>[2x]MNVTVDQSTLAGATRGIVRGGETLKEHRDRLMAATKATGRYAGLKTLELREREPILYNKLFSRLRAGVVDARETAKKIAASPIVEQEGELCFTLYNAAGDSLLTSTGIIIHVGTMGAAIKYMIENNWEANPGVHDKDIFCNNDSLIGNVHPCDIHTIVPIFWEGELIGWVGGVTHVIDTGAVGPGSMATGQVQRFGDGYSITCRKVGANDTLFRDWLHESQRMVRTTRYWMLDERTRIAGCHMIRKLVEEVVAEEGIEAYWKFAYEAVEHGRLGLQARIKAMTIPGTYRQVGFVDVPYAHEDVRVPSDFAKLDTIMHAPCEMTIRRDGTWRLDFEGSSRWGWHTYNAHQVSFTSGIWVMMTQTLIPSEMINDGAAYGTEFRLPKGTWMNPDDRRVAFSYSWHFLVSAWTALWRGLSRSYFGRGYLEEVNAGNANTSNWLQGGGFNQYDEIHAVNSFECAANGTGATAVQDGLSHA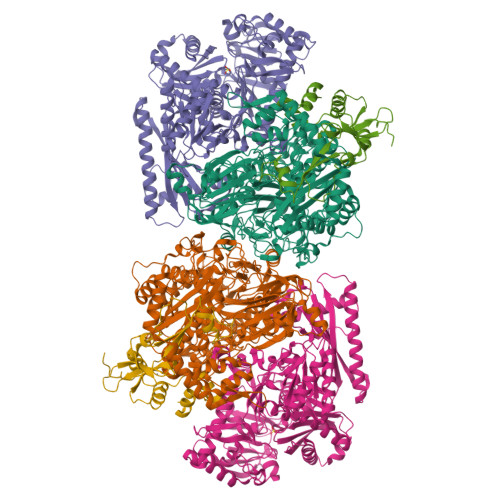AAIWNPEGDMGDMEIWELAEPLVYLGRQIKASSGGSGKYRGGCGFESLRMVWNAKDWTMFFMGNGHISSDWGLMGGYPAASGYRFAAHKTNLKELIASGAEIPLGGDTDPENPTWDAMLPDAQIKRDKQAITTEEMFSDYDLYLNYMRGGPGFGDPLDREPQAVADDINGGYVLERFAGEVYGVVVRKGADGQYGVDEAGTAAARAQIRKDRLAKSVPVSEWMKGEREKILAKDAGTQVRQMFAASFKLGPRFEKDFRTFWSLPDSWTLPEEEIGVPTYGSRYSMDISELPDVHTVQFVEE;>[2x]MHHHHHHSSGMNVPVGHLRNVQVLGIDAGGTMTDTFFVDQDGDFVVGKAQSTPQNEALGLIASSEDGLANWGMSLHEALAQLQTGVYSGTAMLNRVVQRKGLKCGLIVNRGMEDFHRMGRAVQSHLGYAYEDRIHLNTHRYDPPLVPRHLTRGVVERTDMIGTQVIPLREDTARDAARDLIAADAEGIVISLLHSYKNPENERRVRDIVLEEVEKSGKKIPVFASADYYPVRKETHRTNTTILEGYAAEPSRQTLSKISNAFKERGTKFDFRVMATHGGTISWKAKELARTIVSGPIGGVIGAKYLGEVLGYKNIACSDIGGTSFDVALITQGEMTIKNDPDMARLVLSLPLVAMDSVGAGAGSFIRLDPYTRAIKLGPDSAGYRVGVCWKESGIETVTISDCHMVLGYLNPDNFLGGAVKLDRQRSVDAIKAQIADPLGLSVEDAAAGVIELLDSDLRDYLRSMISGKGYSPASFVCFSYGGAGPVHTYGYTEGLGFEDVIVPAWAAGFSAFGCAAADFEYRYDKSLDINMPTETPDTDKEKAAATLQAAWEELTKNVLEEFKLNGYSADQVTLQPGYRMQYRGQLNDLEIESPLAQAHTAADWDQLTDAFNATYGRVYAASARSPELGYSVTGAIMRGMVPIPKPKIPKEPEEGETPPESAKIGTRKFYRKKRWVDAQLYHMESLRPGNRVMGPAVIESDATTFVVPDGFETWLDGHRLFHLREV;>MAYTRSKIVDLVDGKIDPDTLHQMLSTPKDPERFVTYVEILQERMPWDDKIILPLGPKLFIVQQKVSKKWTVRCECGHDFCDWKDNWKLSARVHVRDTPQKMEEIYPRLMAPTPSWQVIREYFCPECGTLHDVEAPTPWYPVIHDFSPDIEGFYQEWLGLPVPERADA[2x]>GAMGKVTHSIHIEKSDTAADTYGFSLSSVEEDGIRRLYVNSVKETGLASKKGLKAGDEILEINNRAADALNSSMLKDFLS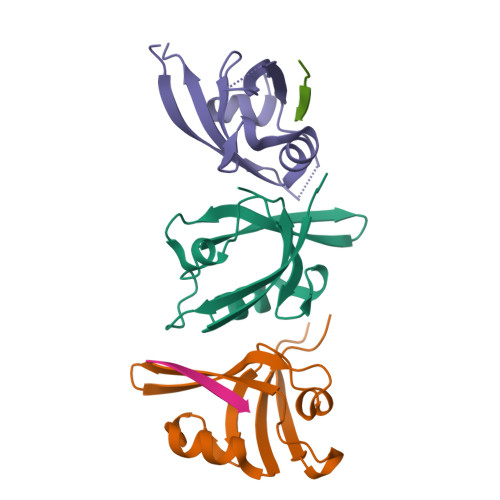QPSLGLLVRTYPEL[3x];>SSRKEYYA[2x]>AGSDPKCTEKEGNRTYNCENLGLREIPDTLPNTTEVLEFSFNFLPTIQNTTFSRLINLIFLDLTRCQINWVHEDTFQSHHQLNTIVLTGNPLIFMAETSLTGPKFLKHLFLTQTGISNLEFIPVHNLENLESLHLGSNHISSINLPENFPTQNLKVLDFQNNAIHYISRKDTNSLEQATNLSLNFNGNDIKGIEPGAFISKIFQSLKFGGSLNLFIIFKGLQNSTLQSLWLGTFEDTDDQYLTSATFEGLCDMSVESINLQKHRFSDLSSSTFRCFTRVQELDLTAAHLNGLPSGIEGMNSLKKLVLNANSFDQLCQINAASFPSLRDLYIKGNMRKLDLGTRCLEKLENLQKLDLSHSDIEASDCCNLQLKNLRHLQYLNLSYNEPLGLEDQAFKECPQLELLDVAFTHLHVKAPHSPFQNLHLLRVLNLSHCLLDTSNQHLLAGLQDLRHLNLQGNSFQDGSISKTNLLQMVGSLEILILSSCNLLSIDQQAFHGLRNVNHLDLSHNSLTGDSMDALSHLKGLYLNMASNNIRIIPPHLLPALSQQSIINLSHNPLDCTCSNIHFITWYKENLHKLEDSEETTCANPPSLRGVKLSDVKLHCGTHMLVPR[8x];>[8x]AGEAWPTHTACRNGNLQVLYQ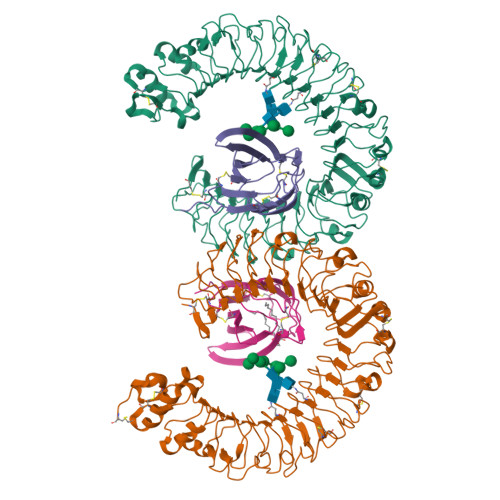SCDPLQDFGFSVDQCARQLKPNINIRFGMVLREDIEQLFLDVALFSKGLSILNFSYPVCEVDLPKFSFCGRRKGEQIYYAGPINNPGFEIPEGDYQVLLELYNQDHATVACANATVLYSARGLVPR DITHIONITE | O4 S2 | 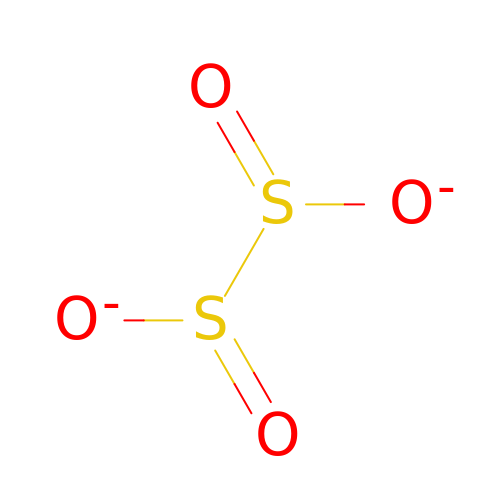GRWZHXKQBITJKP-UHFFFAOYSA-L> SHPALTQL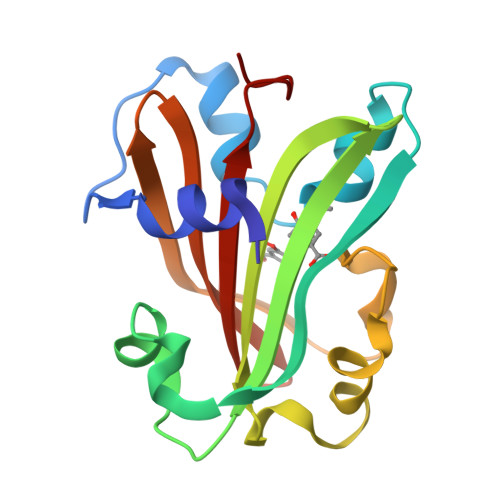RALRYSKEIPALDPQLLDWLLLEDSMTKRFEQQGKTVSVTMIREGFVEQNEIPEELPLLPKESRYWLREILLSADGEPWLAARTVVPVSTLSGPELALQKLGKTPLGRYLFTSSTLTRDFIEIGRDAGLWGRRSRLRLSGKPLLLTELFLPASPLY>GSHMDIQVQVNIDDNGKNFDYTYTVTTESELQKVLNELMDYIKAAGAARVRISITARTSSEAEKFAAILRKVFAELGYNDINVTFDGDTVTVEGQLE[2x]

Top7 is a de novo designed protein consisting of two α-helices and five β-strands. Top7 is a de novo designed protein whose amino acid sequence has no evolutional trace. Because of the lack of an evolutional trace, Top7 is an ideal model protein to study the pure nature of protein structure. The high stability of Top7 also provides a suitable property for protein engineering.

We introduced K42A, Q43A, and K46A mutations and the resulting mutant was named Top7sm1 (sm indicates surface mutations). We mutated these two residues to serine and called this mutant Top7sm2. We scrutinized the crystal packing of Top7sm2 and found Ile68 at β-strand-4 to be a promising site for the mutation. We mutated Ile68 to arginine to introduce repulsive electrostatic force by positive charges and steric hindrance at the interface. We successfully determined the crystal structure of Top7sm2-I68R with a resolution of 1.4 Å. The crystal belongs to the P21 space group, containing two molecules in the asymmetric unit (mol-A and mol-B). As intended, the mutant formed new crystal packing without forming the continuous β-sheet string that was observed in the other Top7 structures, and the R values (R/Rfree: 0.20/0.24) were dropped to a relatively decent range for the resolution. Arg68 slid by each other to avoid steric crash and repulsive electric force, as intended. Although there is no direct contact at K42A, Q43A, and K46A, these mutations seem to prevent steric crash with a neighboring molecule by the removal of the long Lys and Gln side chains. K57S and K58S mutational portions directly form a crystal contact with the Glu28 of a neighboring molecule.>KPIEIIGAPFSKGQPRGGVEKGPAALRKAGLVEKLKETEYNVRDHGDLAFVDVPNDSPFQIVKNPRSVGKANEQLAAVVAETQKNGTISVVLGGDHSMAIGSISGHARVHPDLCVIWVDAHTDINTPLTTSSGNLHGQPVAFLLKELKGKFPDVPGFSWVTPCISAKDIVYIGLRDVDPGEHYIIKTLGIKYFSMTEVDKLGIGKVMEETFSYLLGRKKRPIHLSFAVDGLDPVFTPATGTPVVGGLSYREGLYITEEIYKTGLLSGLDIME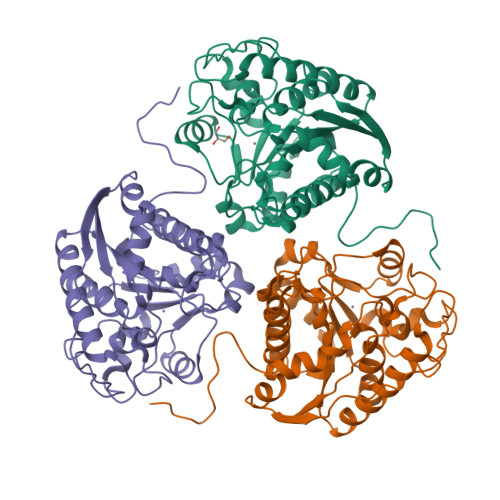VNPTLGKTPEEVTRTVNTAVALTLSCFGTKREGNHKPETDYL[3x]> SNANSYVALYKFLPQENNDLALQPGDRIMLVDDSNEDWWKGKIGDRVGFFPANFVQRVRPGENVWRCC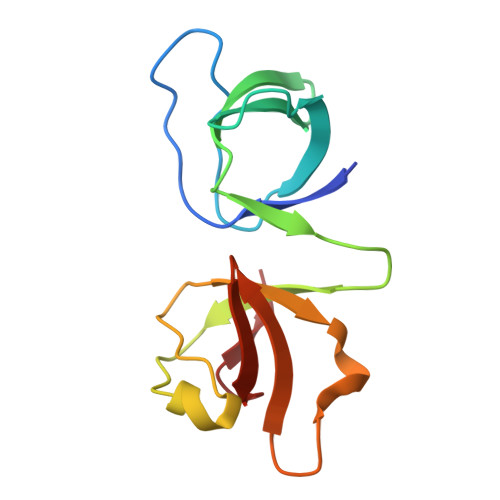QPFSGNKEQGYMSLKENQICVGVGRSKDADGFIRVSSGKKRGLVPVDALTEI>MIGVNRMTEASTYIGTVQDVNGANIRVVLDINTISSLKFVDGQGYRIGQIGSFVRIPIGYINLFGIVSQVGAGAVPDKLLEVEPYGHRWISVQLVGEEGIKKEFERGVSQYPTIGDKVHIVTEPDLKKIYGTQNKKYISLGNIASVDSIPALVNIDTLVTRHSAVLGSTGSGKSTTVTSILQRISDMSQFPSARIIVFDIHGEYAAAFKGKAKVYKVTPSNNELKLSIPYWALTCDEFLSVAFGGLEGSGRNALIDKIYELKLQTLKRQEYEGINEDSLTVDTPIPFSIHKLWFDLYRAEISTHYVQGSHSEENEALLLGEDGNPVQKGDSLKVVPPIYMPHTQAQGATKIYLSNRGKNIRKPLEGLASLLKDPRYEFLFNADDWSVNLDGKTNKDLDALLETWVGSEESISIFDLSGMPSSILDTLIGILIRILYDSLFWSRNQPEGGRERPLLVVLEEAHTYLGKDSRGIAIDGVRKIVKEGRKYGIGMMLVSQRPSEIDSTILSQCGTLFALRMNNSSDRNHVLGAVSDSFEGLMGMLPTLRTGEAIIIGESVRLPMRTIISPPPFGRRPDSLDPDVTAKWSNNRVQGDYKEVLTLWRQKKVRSQRIVENIKRLPVVNEGEMTDMVREMVTSSNILSIGYEADSMTLEIEFNHGLVYQYY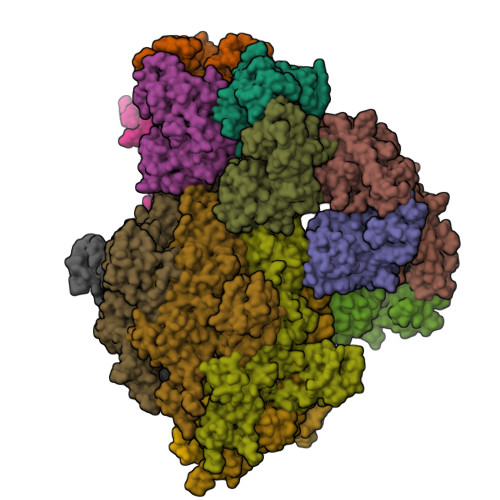DVPETLHTELLAAESHGKFFNSQIKNNYRFSRI[6x];>[9x]MDHSITASYYDTTQQLSLLKHVLSEDKRPIAFIIAAGCPVSIRHNDAPLIPDVAGLTRKISDSFGGNPDSLLMKIIQNLKTTIPNPTIEDILSYIRLLQQIPMSGKIHDVENSVINALEESICELIEEEVNVDLPGNATPYHKIAAWINSINREHQVEIFTTNYDLLMEQALEELNVPYFDGFVGSKRAFFDIRTIEENKLPSRWSKLWKLHGSINWQLDKQTQTIWRGTPSKGCSLIHPSHLKYDQSRKMPYLVMMDQLKLFLNQPSAILITCGYSYKDQHINEVLSQGLQTNPNALIYGLQYDVLENYQEAKDMALKRSNLILLAKDRAIIGKKEGEWKPDPQSSQDNDPLLFFKLGDFQHLASFLEEISQYDWSKQND> MAQGEYLFAITTLILSSAGLYIFANRKAYAWRYVYPGMAGMGLFVLFPLVCTIAIAFTNYSSTNQLTFERAQEVLLDRSWQAGKTYNFGLYPAGDEWQLALSDGETGKNYLSDAFKFGGEQKLQLKETTAQPEGERANLRVITQNRQALSDITAILPDGNKVMMSSLRQ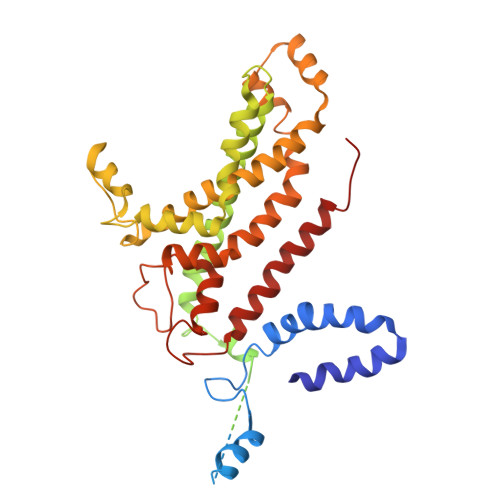FSGTQPLYTLDGDGTLTNNQSGVKYRPNNQIGFYQSITADGNWGDEKLSPGYTVTTGWKNFTRVFTDEGIQKPFLAIFVWTVVFSLITVFLTVAVGMVLACLVQWEALRGKAVYRVLLILPYAVPSFISILIFKGLFNQSFGEINMMLSALFGVKPAWFSDPTTARTMLIIVNTWLGYPYMMILCMGLLKAIPDDLYEASAMDGAGPFQNFFKITLPLLIKPLTPLMIASFAFNFNNFVLIQLLTNGGPDRLGTTTPAGYTDLLVNYTYRIAFEGGGGQDFGLAAAIATLIFLLVGALAIVNLKATRMKFD>[12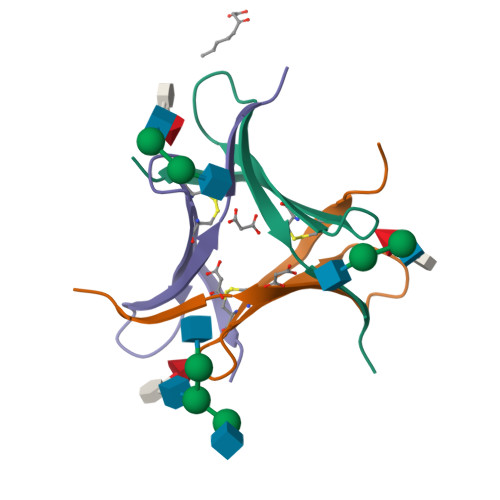x]GAMAPVPVTKLVCDGDTYKCTAYLDFGDGRWVAQWDTNVFHTG>[2x]GMTKTFKTLDDFLGTHFIYTYDNGWEYEWYAKNDHTVDYRIHGGMVAGRWVTD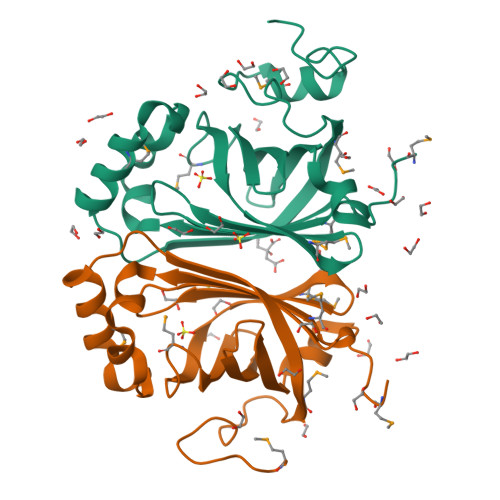QKADIVMLTEGIYKISWTEPTGTDVALDFMPNEKKLHGTIFFPKWVEEHPEITVTYQNEHIDLMEQSREKYATYPKLVVPEFANITYMGDAGQNNEDVISEAPYKEMPNDIRNGKYFDQNYHRLNK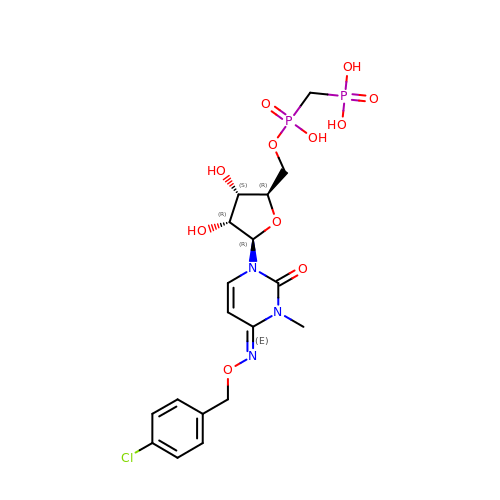[[(2~{R},3~{S},4~{R},5~{R})-5-[(4~{E})-4-[(4-chlorophenyl)methoxyimino]-3-methyl-2-oxidanylidene-pyrimidin-1-yl]-3,4-bis(oxidanyl)oxolan-2-yl]methoxy-oxidanyl-phosphoryl]methylphosphonic acid | C18 H24 Cl N3 O11 P2 | LIVNQTQAYASRSG-UEUWNTQGSA-N> MSSNRVLDLFKPFESFLPEVIAPERKVPYNQKLIWTGVSLLIFLILGQIPLYGIVSSETSDPLYWLRAMLASNRGTLLELGVSPIITSSMIFQFLQGTQLLQIRPESKQDRELFQIAQKVCAIILILGQALVVVMTGNYGAPSDLGLPICLLLIFQLMFASLIVMLLDELLSKGYGLGSGISLFTATNIAEQIFWRAFAPTTVNSGRGKEFEGAVIAFFHLLAVRKDKKRALVEAFYRTNLPNMFQVLMTVAIFLFVLYLQGFRYELPIRSTKVRGQIGIYPIKLFYTSNTPIMLQSALTSNIFLISQILFQKYPTNPLIRLIGVWGIRPGTQGPQMALSGLAYYIQPLMSLSEALLDPIKTIVYITFVLGSCAVFSKTWIEISGTSPRDIAKQFKDQGMVINGKRETSIYRELKKIIPTAAAFGGATIGALSVGSDLLGTLGSGASILMATTTIYGYYEAAAKEGGFTKNLVPGFSDLM;> MSSPTPPGGQRTLQKRKQGSSQKVAASAPKKNTNSNNSILKIYSDEATGLRVDPLVVLFLAVGFIFSVVALHVISKVAGKLF;> MARASEKGEEKKQSNNQVEKLVEAPVEFVREGTQFLAKCKKPDLKEYTKIVKAVGIGFIAVGIIGYAIKLIHIPIRYVIV;> MPTNYEYDEASETWPSFILTGLLMVVGPMTLLQIYQIFFGANAEDGNSGKSKEFNEEVFKNLNEE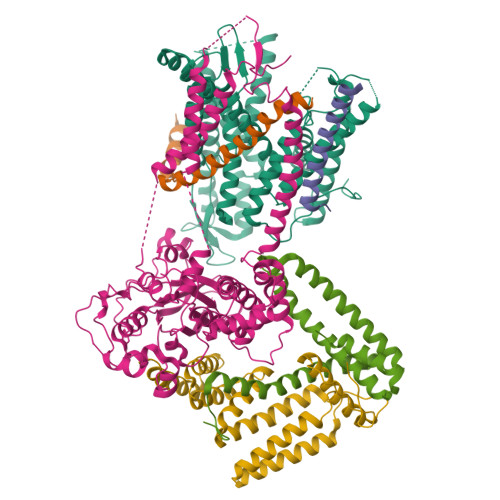YTSDEIKQFRRKFDKNSNKKSKIWSRRNIIIIVGWILVAILLQRINSNDAIKDAATKLFDPYEILGISTSASDRDIKSAYRKLSVKFHPDKLAKGLTPDEKSVMEETYVQITKAYESLTDELVRQNYLKYGHPDGPQSTSHGIALPRFLVDGSASPLLVVCYVALLGLILPYFVSRWWARTQSYTKKGIHNVTASNFVSNLVNYKPSEIVTTDLILHWLSFAHEFKQFFPDLQPTDFEKLLQDHINRRDSGKLNNAKFRIVAKCHSLLHGLLDIACGFRNLDIALGAINTFKCIVQAVPLTPNCQILQLPNVDKEHFITKTGDIHTLGKLFTLEDAKIGEVLGIKDQAKLNETLRVASHIPNLKIIKADFLVPGENQVTPSSTPYISLKVLVRSAKQPLIPTSLIPEENLTEPQDFESQRDPFAMMSKQPLVPYSFAPFFPTKRRGSWCCLVSSQKDGKILQTPIIIEKLSYKNLNDDKDFFDKRIKMDLTKHEKFDINDWEIGTIKIPLGQPAPETVGDFFFRVIVKSTDYFTTDLDITMNMKVRDSPAVEQVEVYSEEDDEYSTDDDETESDDESDASDYTDIDTDTEAEDDESPE;> MSEFNETKFSNNGTFFETEEPIVETKSISVYTPLIYVFILVVSLVMFASSYRKKQAKKISEQPSIFDENDAHDLYFQIKEMSENEKIHEKVLKAALLNRGAESVRRSLKLKELAPQINLLYKNGSIGEDYWKRFETEVKLIELEFKDTLQEAERLQPGWVQLFVMVCKEICFNQALSRRYQSILKRKEVCIKEWELKINNDGRLVN;> MVTLEYNANSKLITASDAVVALSTETNIDQINVLTTSLIGETNPNFTPQPNEALSKMIKGLFESGMKNLQQKKLNEALKNVSLAIEMAQRKRAPWEAFAIQLPELHFMLRSKIDLCLILGKHLEALQDLDFLLGTGLIQPDVFVRKADCLLKLRQWEEARATCERGLALAPEDMKLRALLIETARNLAEYNGE5-methyl-1H-tetrazole | C2 H4 N4 | 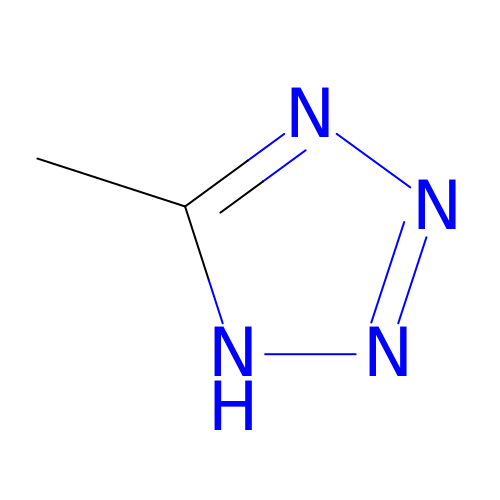XZGLNCKSNVGDNX-UHFFFAOYSA-N> MSEQYSEINTDTLERVTEIFKALGDYNRIRIMEALSVSEASVGHISHQLNLSQSNVSHQLKLLKSVHLVKAKRQGQSMIYSLDDIHVATMLKQAIHHANH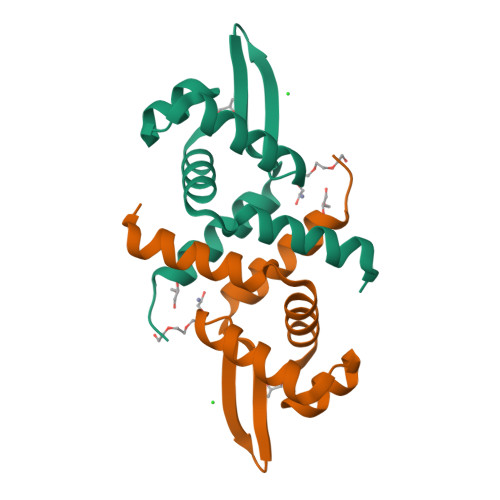PKESGL> MAMHPRKDWYELTRATNWTPSYVTEEQLFPERMSGHMGIPLEKWESYDEPYKTSYPEYVSIQREKDAGAYSVKAALERAKIYENSDPGWISTLKSHYGAIAVGEYAAVTGEGRMARFSKAPGNRNMATFGMMDELRHGQLQLFFPHEYCKKDRQFDWAWRAYHSNEWAAIAAKHFFDDIITGRDAISVAIMLTFSFETGFTNMQFLGLAADAAEAGDYTFANLISSIQTDESRHAQQGGPALQLLIENGKREEAQKKVDMAIWRA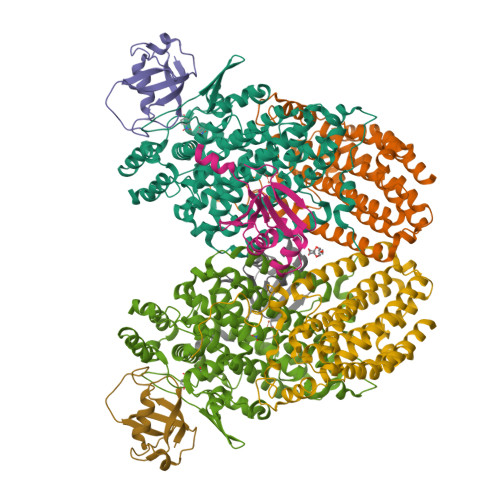WRLFAVLTGPVMDYYTPLEDRSQSFKEFMYEWIIGQFERSLIDLGLDKPWYWDLFLKDIDELHHSYHMGVWYWRTTAWWNPAAGVTPEERDWLEEKYPGWNKRWGRCWDVITENVLNDRMDLVSPETLPSVCNMSQIPLVGVPGDDWNIEVFSLEHNGRLYHFGSEVDRWVFQQDPVQYQNHMNIVDRFLAGQIQPMTLEGALKYMGFQSIEEMGKDAHDFAWADKCKPAMKKSA;> MSFESKKPMRTWSHLAEMRKKPSEYDIVSRKLHYSTNNPDSPWELSPDSPMNLWYKQYRNASPLKHDNWDAFTDPDQLVYRTYNLMQDGQESYVQSLFDQFNEREHDQMVREGWEHTMARCYSPLRYLFHCLQMSSAYVQQMAPASTISNCCILQTADSLRWLTHTAYRTHELSLTYPDAGLGEHERELWEKEPGWQGLRELMEKQLTAFDWGEAFVSLNLVVKPMIVESIFKPLQQQAWENNDTLLPLLIDSQLKDAERHSRWSKALVKHALENPDNHAVIEGWIEKWRPLADRAAEAYLSMLSSD;> MSAFPVHAAFEKDFLVQLVVVDLNDSMDQVAEKVAYHCVNRRVAPREGVMRVRKHRSTELFPRDMTIAESGLNPTEVIDVVFEE;> MSTLADQALHNNNVGPIIRAGDLVEPVIETAEIDNPGKEITVEDRRAYVRIAAEGELILTRKTLEEQLGRPFNMQELEINLASFAGQIQADEDQIRFYFDKTM[1-{4-[6-amino-4-(trifluoromethyl)pyridin-3-yl]-6-(morpholin-4-yl)-1,3,5-triazin-2-yl}-3-(chloromethyl)azetidin-3-yl]methanol | C18 H21 Cl F3 N7 O2 | 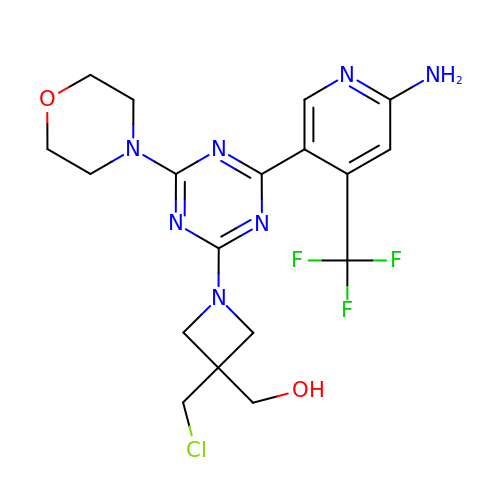LKZNXFAHMCIKNB-UHFFFAOYSA-N structures of the Mep2 transceptors from S. cerevisiae and C. albicans. function as ammonium receptors/sensors in fungal development. a central channel for the transport of ammonium. non-phosphorylated, with channels that are closed on the cytoplasmic side.

The channels of phosphorylation-mimicking mutants of C. well-defined electronegative pocket that is solvent accessible. in turn might cause substantial conformational changes within the CTR. residues has only undergone a slight shift compared with the WT protein. WT CaMep2, the DD mutant and phosphorylated protein (S453J). from Asp452 and Asp453, presumably to avoid electrostatic repulsion. generates conformational changes in the conserved part of the CTR. Leu427 to Asp438 unravels during the simulations to a disordered state. remainder of the protein is not affected.

> MSGQFTGTGTGGDVFKVDLNEQFDRADMVWIGTASVLVWIMIPGVGLLYSGISRKKHALSLMWAALMAACVAAFQWFWWGYSLVFAHNGSVFLGTLQNFCLKDVLGAPSIVKTVPDILFCLYQGMFAAVTAILMAGAGCERARLGPMMVFLFIWLTVVYCPIAYWTWGGNGWLVSLGALDFAGGGPVHENSGFAALAYSLWLGKRHDPVAKGKVPKYKPHSVSSIVMGTIFLWFGWYGFNGGSTGNSSMRSWYACVNTNLAAATGGLTWMLVDWFRTGGKWSTVGLCMGAIAGLVGITPAAGYVPVYTSVIFGIVPAIICNFAVDLKDLLQIDDGMDVWALHGVGGFVGNFMTGLFAADYVAMIDGTEIDGGWMNHHWKQLGYQLAGSCAVAAWSFTVTSIILLAMDRIPFLRIRLHEDEEMLGTDLAQIGEYAYYADDDPETNPYVLEPIDDTTISQPLPHIDGVADGSSNNDSGEAKNHHHHHH>[2x]MSMLGERRRGLTDPEMAAVILKALPEAPLDGNNKMGYFVTPRWKRLTEYEALTVYAQPNADWIAGGLDWGDWTQKFHGGRPSWGNETTELRTVDWFKHRDPLRRWHAPYVKDKAEEWRYTDRFLQGYSADGQIRAMNPTWRDEFINRYWGAFLFNEYGLFNAHSQGAREALSDVTRVSLAFWGFDKIDIAQMIQLERGFLAKIVPGFDESTAVPKAEWTNGEVYKSARLAVEGLWQEVFDWNESAFSVHAVYDALFGQFVRREFFQRLAPRFGDNLTPFFINQAQTYFQIAKQGVQDLYYNCLGDDPEFSDYNRTVMRNWTGKWLEPTIAALRDFMGLFAKLPAGTTDKEEITASLYRVVDDWIEDYASRIDFKADRDQIVKAVLAGLK;>[2x]MALSTATKAATDALAANRAPTSVNAQEVHRWLQSFNWDFKNNRTKYATKYKMANETKEQFKLIAKEYARMEAVKDERQFGSLQDALTRLNAGVRVHPKWNETMKVVSNFLEVGEYNAIAATGMLWDSAQAAEQKNGYLAQVLDEIRHTHQCAYVNYYFAKNGQDPAGHNDARRTRTIGPLWKGMKRVFSDGFISGDAVECSLNLQLVGEACFTNPLIVAVTEWAAANGDEITPTVFLSIETDELRHMANGYQTVVSIANDPASAKYLNTDLNNAFWTQQKYFTPVLGMLFEYGSKFKVEPWVKTWNRWVYEDWGGIWIGRLGKYGVESPRSLKDAKQDAYWAHHDLYLLAYALWPTGFFRLALPDQEEMEWFEANYPGWYDHYGKIYEEWRARGCEDPSSGFIPLMWFIENNHPIYIDRVSQVPFCPSLAKGASTLRVHEYNGQMHTFSDQWGERMWLAEPERYECQNIFEQYEGRELSEVIAELHGLRSDGKTLIAQPHVRGDKLWTLDDIKRLNCVFKNPVKAFN;>MAKLGIHSNDTRDAWVNKIAQLNTLEKAAEMLKQFRMDHTTPFRNSYELDNDYLWIEAKLEE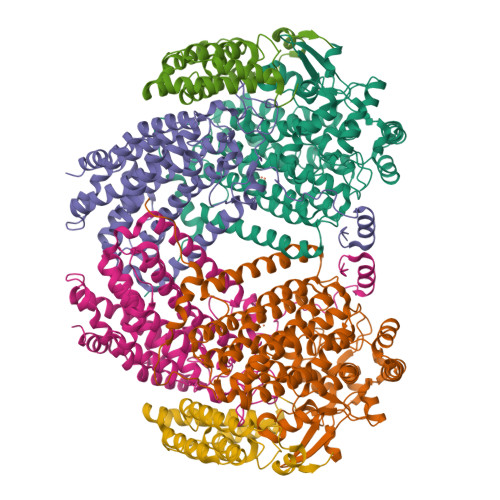KVAVLKARAFNEVDFRHKTAFGEDAKSVLDGTVAKMNAAKDKWEAEKIHIGFRQAYKPPIMPVNYFLDGERQLGTRLMELRNLNYYDTPLEELRKQRGVRVVHLQSPH[2x]>[2x]MGSSHHHHHHSSGRENLYFQGMPKLILASTSPWRRALLEKL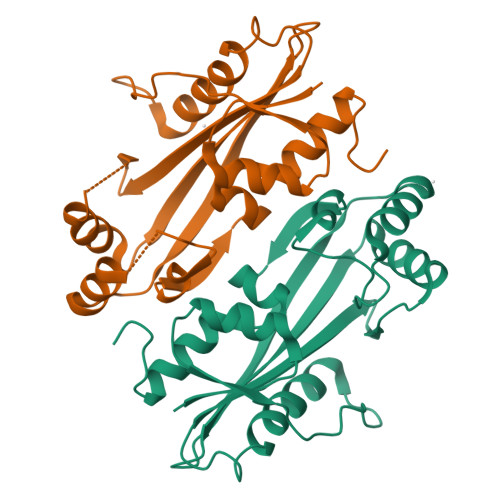QISFECAAPEVDETPRSDESPRQLVLRLAQEKAQSLASRYPDHLIIGSAQVCVLDGEITGKPLTEENARLQLRKASGNIVTFYTGLALFNSANGHLQTEVEPFDVHFRHLSEAEIDNYVRKEHPLHCAGSFKSEGFGITLFERLEGRDPNTLVGLPLIALCQMLRREGKNPLMG>[2x]MKCRVVTTTGTADWSVRESFNNYLEGPIANGAAYKYHGGIEVRDGVETTGTKSAREFTWPVLGSEEGAVKLGGGVHWTGHNHYSGDDESQAPDNFILDLDFSNPTVKFDGNEGTLLV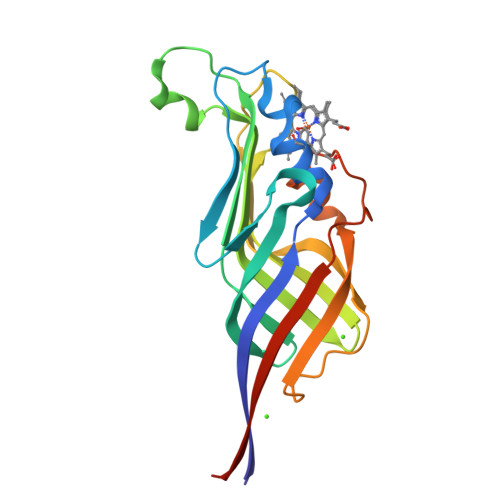DFKSREFVDTKTVADFLTGTQAELATITFDEPIDLTQENVTVTGQTKLTATGVDVMGTFYPEGEALAPITLNLTNEVVLEHHHHHH> NGEI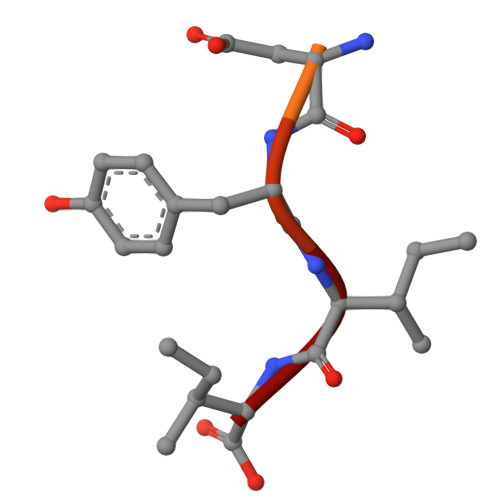QDDYII Cyclic GMP-AMP (cGAMP) synthase (cGAS) is essential for the host defense against cytosolic double-stranded (ds)DNA arising from various maladies (e.g., pathogen invasion, ionizing irradiation, and genotoxic chemicals). Upon directly binding to and dimerizing on dsDNA, cGAS cyclizes ATP and GTP into 2′−5′/3′−5′-linked cGAMP, a unique metazoan second messenger for initiating type-I interferon (IFN-I)-mediated inflammatory responses. cGAS is central to antitumor immunity, host defense against an array of pathogens, and regulating autoimmunity. Here, we resolve these numerous fundamental mechanistic questions in innate immunology and present a unifying catalytic mechanism of cGAS. Finally, we reveal how mouse cGAS achieves more stringent substrate selectivity and higher catalytic efficiency than the human enzyme. Together, we set forth a unifying catalytic mechanism of cGAS in which dsDNA-binding pre-organizes the active site into a rigid yet adaptable lock for two sets of keys (substrates and intermediate) necessary to specifically synthesize 2′−5/3′−5′-cGAMP.

To test functional implications, we soaked QN-mcGAScat•dsDNA with inosine triphosphate (ITP)/GTP or ATP/ITP. In the ITP/GTP-soaked structure, judged by the electron density for the -NH2 of GTP, it appeared that ITP and GTP bind at Site-1 and Site-2, respectively. Moreover, the ATP/ITP-soaked structure suggested that ATP and ITP are bound at Site-1 and Site-2, respectively; the carboxyl oxygen of ITP appeared to accept a H-bond from Ser366 as seen from GTP, and ATP fails to bind stably at Site-2 in all known structures (see also below for the pppGpA-bound structure). These results support the idea that the -NH2 of GTP is disfavored at Site-1 while the -NH2 of ATP at Site-1 provides a favorable interaction for site-specific ATP/GTP binding. E, F QN-mcGAScat•dsDNA bound to ITP/GTP (E) and ATP/ITP (F). Consistent with the idea that GTP is disfavored over ITP at Site-1, mcGAScat was more active toward ITP/ITP vs. GTP/GTP.

>[2x]GTGPDKLKKVLDKLRLKRKDISEAAETVNKVVERLLRRMQKRESEFKGVEQLNTGSYYEHVKISAPNQFNVMFKLEVPRIELQEYYETGAFYLVKFKRIPRGNPLSHFLEGEVLSATKMLSKFRKIIKEEVKEIKDIDVSVEKEKPGSPAVTLLIRNPEEISVDIILALESKGSWPISTKEGLPIQGWLGTKVRTNLRREPFYLVPKNAKDGNSFQGETWRLSFSHTEKYILNNHGIEKTCCESSGAKCCRKECLKLMKYLLEQLKKEFQELDAFCSYHVKTAIFHMWTQDPQDSQWDPRNLSSCFDKLLAFFLECLRTEKLDHYFIPKFNLFSQELIDRKSKEFLSKKIEYERNNGFPIFDKL>MQVEANSERRVKILGIDRSENSPVLTYMETEDDPNFRNSKLAAAPHTVHMMDSGFLAINRQCLVKGKAILAREPKSSNEHMIDDLPKHAHDQHTLSILRDFIDQLKLHNVYEINFYDPLDSSGKLAVIPMLIALWKCMLASETDICDQEVLKSIMNSVIAKFELQIPCKNAVIDATLSGSREEVHIIAEDGSLENSNGTTEHFNKKHDLVFVKTDLHPEDFTPQMFPSQAKAKLLRDAFNNEEDEDTFPDILVPAYMTAHSKNRVRQEDYTCLEVEFDSQVALEKLMNEHEQVEGFEVQQGGILVALKKDSFFDDELIEKIAIAIATESRQSVSSVSFDLLKLGPGASLVTLANSRRFEPECRVVLQIEVKPVSPGETSSEGISDEHHYEEYDEDDIMEEEEAPSARQDDTYD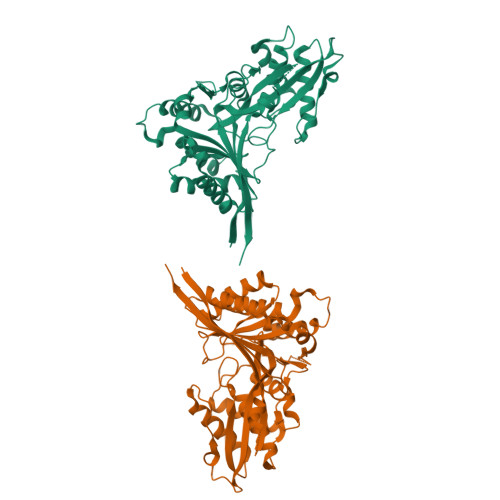EDEE[2x]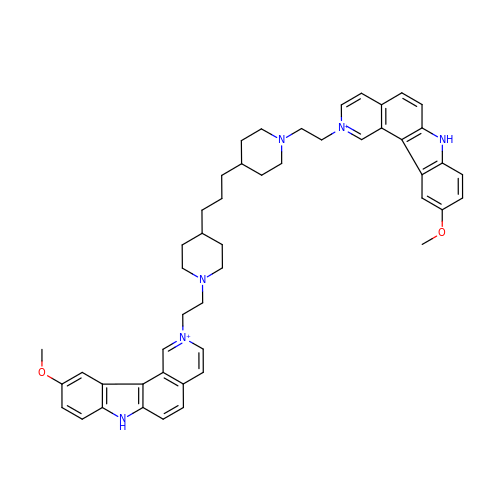1,3-DI[[[10-METHOXY-7H-PYRIDO[4,3-C]CARBAZOL-2-IUMYL]-ETHYL]-PIPERIDIN-4-YL]-PROPANE | C49 H56 N6 O2 | OAPSNAJHSNYHAG-UHFFFAOYSA-P> QFAKPEDAVKYRQSALTLMASHFGRMTPVVKGQAPYDAAQIKANVEV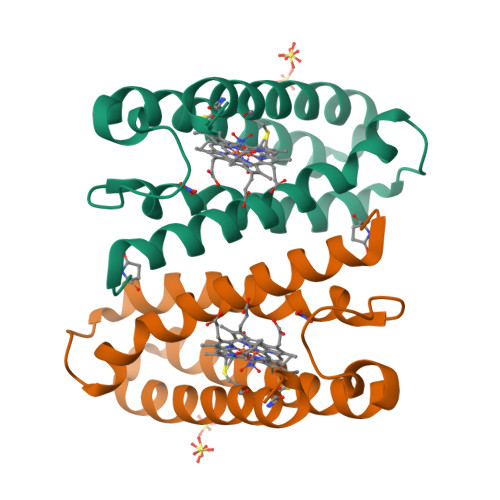LKTLSALPWAAFGPGTEGGDARPEIWSDAASFKQKQQAFQDNIVKLSAAADAGDLDKLRAAFGDVGASCKACHDAYAKKK> MVDFYYLPGSSPCRS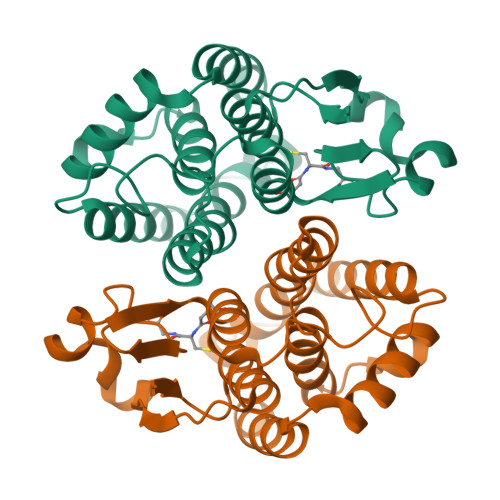VIMTAKAVGVELNKKLLNLQAGEHLKPEFLKINPQHTIPTLVDNGFALWESRAIQVYLVEKYGKTDSLYPKCPKKRAVINQRLYFDMGTLYQSFANYYYPQVFAKAPADPEAFKKIEAAFEFLNTFLEGQDYAAGDSLTVADIALVATVSTFEVAKFEISKYANVNRWYENAKKVTPGWEENWAGCLEFKKYFE> GPMGNGMNKILPGLYIGNFKDARDAEQLSKNKVTHILSV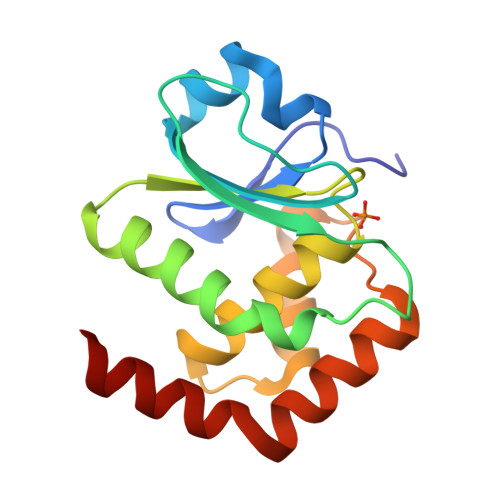HDSARPMLEGVKYLCIPAADSPSQNLTRHFKESIKFIHECRLRGESCLVHSLAGVARSVTLVIAYIMTVTDFGWEDALHTVRAGRSCANPNVGFQRQLQEFEKHEVHQYRQWLKEEYG> NYMGNPWTEYMAKYDIEEVHGSGIRVDLGEDAEVAGTQYRLPSGKCPVFGKGIIIENSNTTFLKPVATGNQDLKDGGFAFPPTNPLISPMTLNGMRDFYKNNEYVKNLDELTLCSRHAGNMNPDNDKNSNYKYPAVYDYNDKKCHILYIAAQENNGPRYCNKDQSKRNSMFC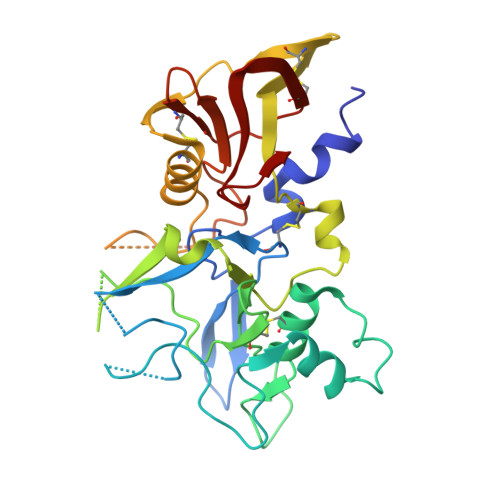FRPAKDKLFENYTYLSKNVVDNWEEVCPRKNLENAKFGLWVDGNCEDIPHVNEFSANDLFECNKLVFELSASDQPKQYEQHLTDYEKIKEGFKNKNASMIKSAFLPTGAFKADRYKSHGKGYNWGNYNRETQKCEIFNVKPTCLINNSSYIATTALSHPIEVE>ETGDKPLGETGTTGFQICKNALKLPVLEVLPGGGWDNLRNVDMGRVMDLTYTNCKTTEDGQYIIPDEVYTIPQKESNLEMNSEVLESWMNYQSTTSLSINTELALFSRVNGKFSTEFQRMKTLQVKDQAVTTRVQVRNRIYTVKTTPTSELSLGFTKALMDICDQLEKNQTKMATYLAELLILNYGTHVITSVDAGAALVQEDHVRSSFLLDNQNSQNTVTASAGIAFLNIVNFKVETDYISQTSLTKDYLSNRTNSRVQSFGGVPFYPGITLETWQKGITNHLVAIDRAGLPLHFFIKPDKLPGLPGPLVKKLSKTVETAVRHYYTFNTHPGCTNVDSPNFNFQANMDDDSCDAKVTNFTFGGVYQECTELSGDVLCQNLEQKNLLTGDFSCPPGYSPVHLLSQTHEEGYSRLECKKKCTLKIFCKTVCEDVFRVAKAEFRAYWCVAAGQVPDNSGLLFGGVFTDKTINPMTNAQSCPAGYIPLNLFESLKVCVSLDYELGFKFSVPFGGFFSCIMGNPLVNSDTAKDVRAPSLKKCPGGFSQHLAVISDGCQVSYCVKAGIFTGGSLLPVRLPPYTKPPLMSQVATNTVIVTNSETARSWIKDPQTNQWKLGEPLELRRAMTVIHGDSNGM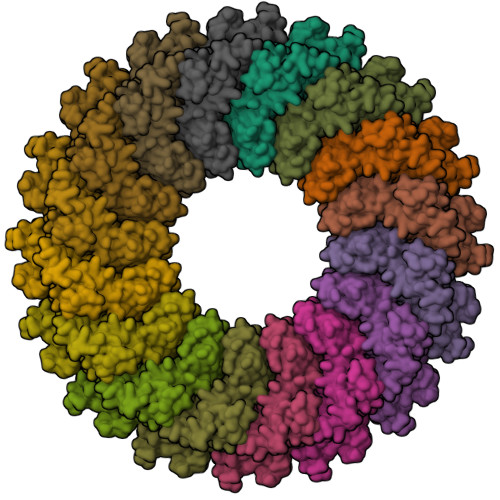SGGGTKTETSQVAPA[16x]>MAQHLLHGTLHATIYEVDALHGGGVRQGFLGKILANVEETIGVGKGETQLYATIDLQKARVGRTRKIKNEPKNPKWYESFHIYCAHLASDIIFTVKDDNPIGATLIGRAYIPVDQVINGEEVDQWVEILDNDRNPIQGGSKIHVKLQYFHVEEDRNWNMGIKSAKFPGVPYTFFSQRQGCKVSLYQDAHIPDNFVPRIPLAGGKNYEPQRCWEDIFDAISNAKHLIYITGWSVYAEIALVRDSRRPKPGGDVTIGELLKKKASEGVRVLLLVWDDRTSVDVLKKDGLMATHDEETENFFRGSDVHCILCPRNPDDGGSIVQSLQISTMFTHHQKIVVVDSEMPSRGGSEMRRIVSFVGGIDLCDGRYDTPFHSLFRTLDTVHHDDFHQPNFTGAAITKGGPREPWHDIHSRLEGPIAWDVMYNFEQRWSKQGGKDILVKLRDLSDIIITPSPVMFQEDHDVWNVQLFRSIDGGAAAGFPESPEAAAEAGLVSGKDNIIDRSIQDAYIHAIRRAKDFIYVENQYFLGSSFAWAADGITPEDINALHLIPKELSLKIVSKIEKGEK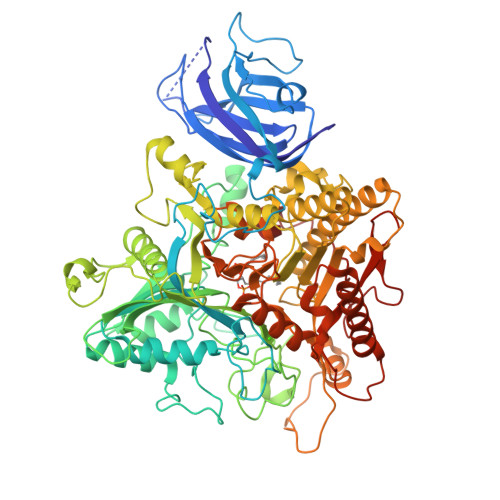FRVYVVVPMWPEGLPESGSVQAILDWQRRTMEMMYKDVIQALRAQGLEEDPRNYLTFFCLGNREVKKDGEYEPAEKPDPDTDYMRAQEARRFMIYVHTKMMIVDDEYIIIGSANINQRSMDGARDSEIAMGGYQPHHLSHRQPARGQIHGFRMSLWYEHLGMLDETFLDPSSLECIEKVNRISDKYWDFYSSESLEHDLPGHLLRYPIGVASEGDITELPGFEFFPDTKARILGTKSDYLPPILTT[2x]>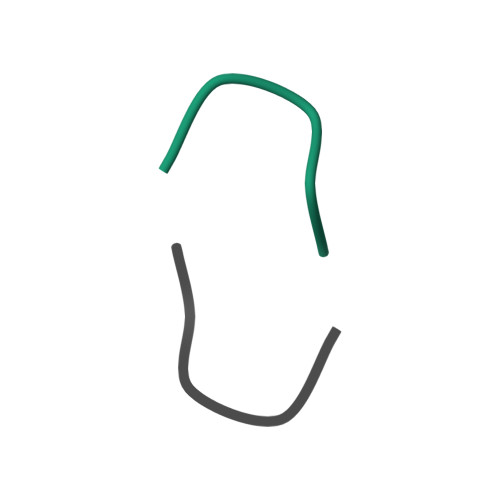 PSEIRPSEIR> GDCEMKRTTLDSPLGKLELSGCEQGLHEIIFLG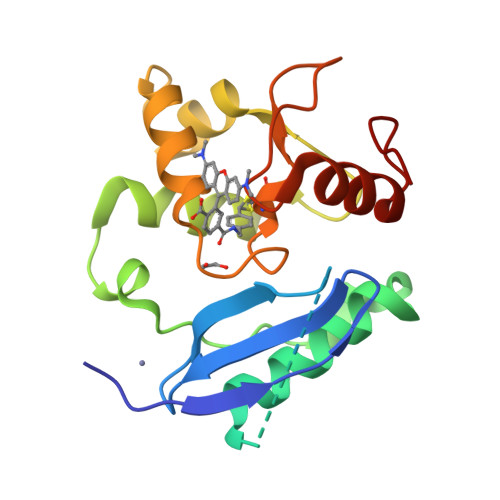KGTSAADAVEVPAPAAVLGGPEPLMQATAWLNAYFHQPEAIEEFPVPALHHPVFQQESFTRQVLWKLLKVVKFGEVISYSHLAALAGNPAATAAVKTALSGNPVPILIPCHRVVQGDLDVGGYEGGLAVKEWLLAHEGHRLGKR>[5x]VSPPPPIADEPLTVNTGIYLIECYSLDDKAETFKVNAFLSLSWKDRRLAFDPVRSGVRVKTYEPEAIWIPEIRFVNVENARDADVVDISVSPDG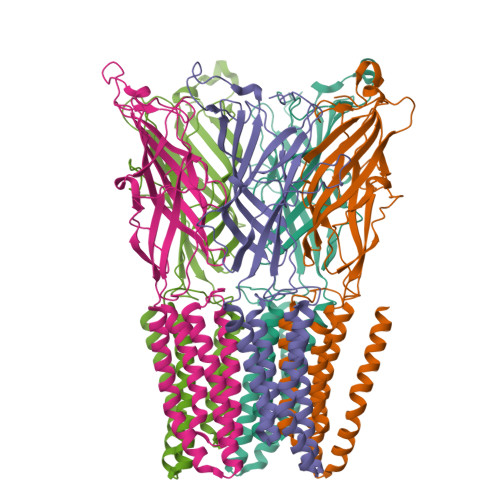TVQYLERFSARVLSPLDFRRYPFDSQTLHIYLIVRSVDTRNIVLAVDLEKVGKNDDVFLTGWDIESFTAVVKPANFALEDRLESKLDYQLRISRQYFSYIPNIILPMLFILFISWTAFWSTSYEANVTLVVSTLIAHIAFNILVETNLPKTPYMTYTGAIIFMIYLFYFVAVIEVTVQHYLKVESQPARAASITRASRIAFPVVFLLANIILAFLFF> MRVRIRGIYATALTYLFLKNGFEIVQQTPQIAERFFMDIIRSPADVTVKDGIDKGEIVSVGEDIYNFMRSIFKYSPIWRSPIKLYSVVSTEDCKFMNFIVEPCLSEGLVIKPPVEGKIILSSPRAVGKFAMVWKGDGRTFFSEHIDERDSQRLLSVSIPFNKKGYNVKWRSNAAMATTAELKEELENLTMRYSYNDFREQGEDFLKVTLSLEDKLFLDDIRSLVINTMKFHHMLKMTYSNEVDIEEGKVNPSPEKLLTSLIGDNMIEAIEHVKPNGKRVLLKGGTIVQKEIGRDYYWLKIRREFKSGGIYDGLNLKIEDGDYDLVELDSRNWYQIHRYHDRNNNLKGLYVNISTPPELLKNRIRYLDLEVDVVKVNNTVNIIDLEELEANKPILGEFLYKKALEIAQNIKDKLNEDKI

Here, we report two X-ray crystallographic structures of RNase G/E-like–DUF402 hybrid proteins from Pyrococcus furiosus and Sulfolobus acidocaldarius, at 2.1 and 2.0 Å, respectively. Our study provides structural and functional evidence that the archaeal DUF402 domain acts as an RNase, whereas the G/E-like domain is catalytically inactive, and may serve as a regulatory and substrate recognition subunit. Finally, in vivo experiments in Haloferax volcanii suggest that this RNase participates in the maturation of pre-16S rRNA.

The structure of the SaRNase W protein was solved to 2.0 Å by molecular replacement using the PfRNase W protein as a model. Two magnesium ions, two phosphate ions and two bound dinucleotides from the co-purified RNA are visible in the PfRNase W structure and only two magnesium ions in the SaRNase W structure. Although the overall structures of both RNase W proteins are similar with 27.5% sequence identity, they can be superimposed with a 5.6 Å root mean square deviation (rmsd) over all 400 C-alpha atom pairs. The domain orientations only vary slightly between both proteins; each domain can be superposed individually with an ∼1 Å rmsd on equivalent residues (across 58 atom pairs for N-terminal domain, across 6 atom pairs for S1 domain, across 53 atom pairs for 5′-sensor domain, across 33 atom pairs for α helical bundle domain and across 110 atom pairs for DUF402 domain). In the PfRNase W structure with a 5′-phosphate dinucleotide bound in the 5′-sensor domain, the central domain with R10 completes the recognition of the 5′-phosphate through a double hydrogen bond interaction. In the SaRNase W structure, the position of a bound 5′-phosphate (modeled in Figure 6B) would be 4.5 Å away from R10 (R4 in SaRNase W). Instead, R10 makes an H bond with S171 from the 5′-sensor domain. We hypothesize that the difference in conformation arises from binding and recognition of a 5′-phosphate RNA, which locks the 5′-sensor and S1 domains in a productive conformation through the specific recognition of the 5′-phosphate by R10.6-BROMO-9-AMINO-N-ETHYL(DIAMINOMETHYL)ACRIDINE-4-CARBOXAMIDE | C18 H21 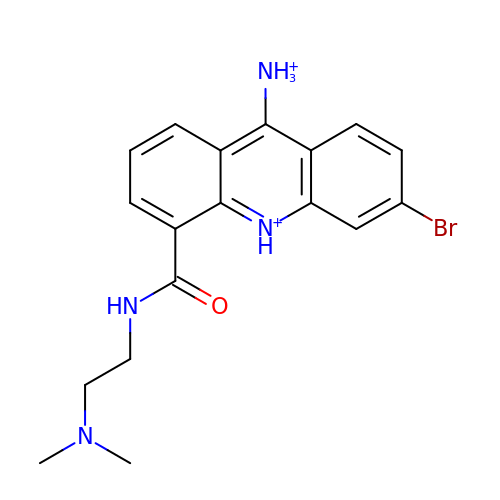Br N4 O | HBKKAYCZISIMFL-UHFFFAOYSA-P>ASMTGGQQMGRDEAGITGTWYNQLGSTFIVTAGADGALTGTYESAVGNAESRYVLTGRYDSAPATDGSGTALGWTVAWKNNYRNAHSATTWSGQYVGGAEARINTQWLLTAGTTEANAWKSTLVGHDTFTKVKPSAASIDAAKKAGVNNGN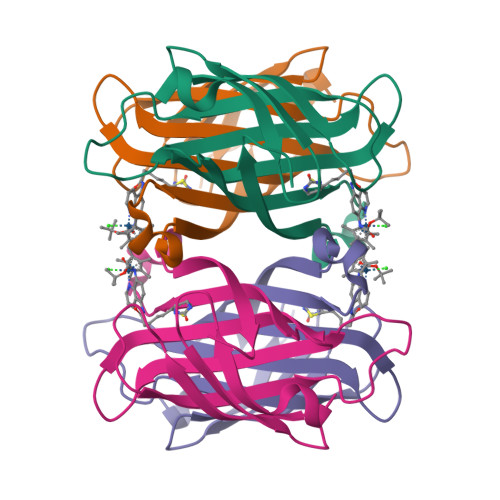PLDAVQQ[4x]4-aminocinnoline-3-carboxamide 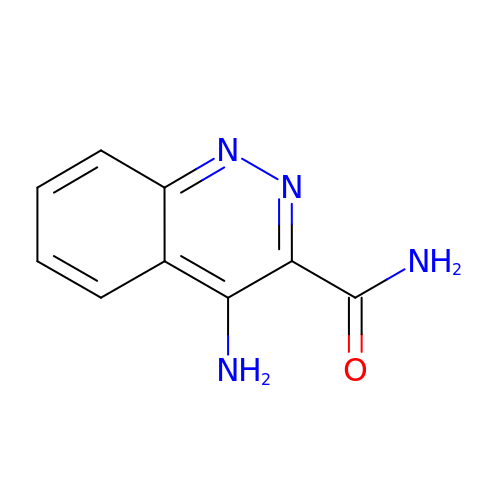| C9 H8 N4 O | FCYPWSQPDXUBPV-UHFFFAOYSA-N>MSETAPLPSASSALEDKAASAPVVGIIMGSQSDWETMRHADALLTELEIPHETLIVSAHRTPDRLADYARTAAERGLNVIIAGAGGAAHLPGMCAAWTRLPVLGVPVESRALKGMDSLLSIVQMPGGVPVGTLAIGASGAKNAALLAASILALYNPALAARLETW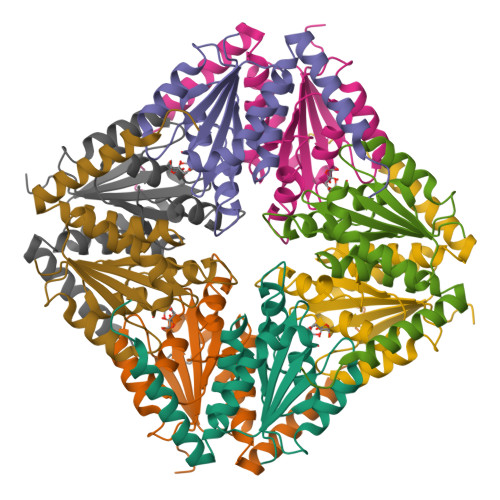RALQTASVPNSPITEDK[2x]>[2x]GEPSLGLVAKDSPAEKGGLKVGDTVVSVNGESISLWSEFVSFIENNPGKPLELI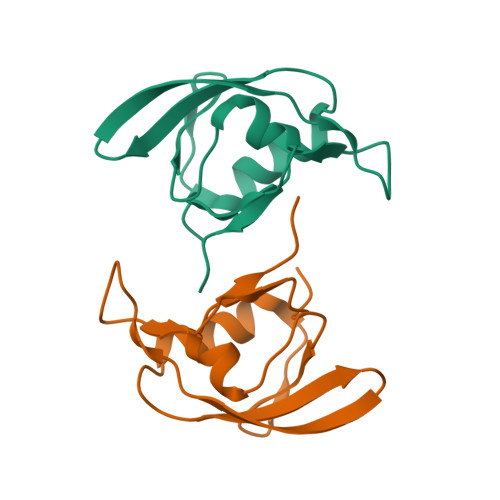VARDGYQQPLVVTPEANERDRTIGYLGISPAFQ> QYPIINFTTAGATVQSYTNFIRAVRGRLTTGADVRHEIPVLPNRVGLPINQRFILVELSNHAELSVT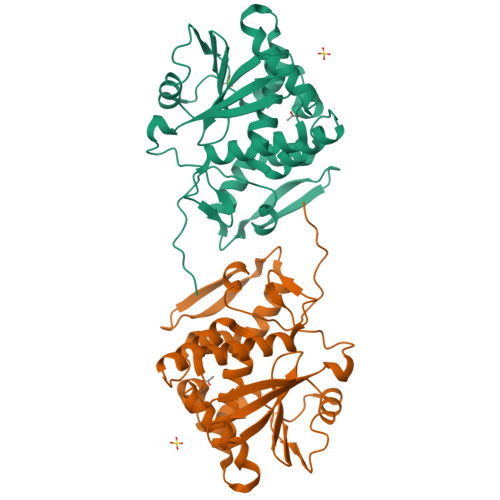LALDVTNAYVVGYRAGNSAYFFHPDNQEDAEAITHLFTDVQNRYTFAFGGAYDRLEQLAGNLRENIELGNGPLEEAISALYYYSTGGTQLPTLARSFIICIQMISEAARFQYIEGEMRTRIRYNRRSAPDPSVITLENSWGRLSTAIQESNQGAFASPIQLQRRNGSKFSVYDVSILIPIIALMVYRCAPPPSSQF>[2x]GPHMSDHKFLTQAVEEAYKGVDCGDGGPFGAVIVHNNEVVASCHNMVLKYTDPTAHAEVTAIREACK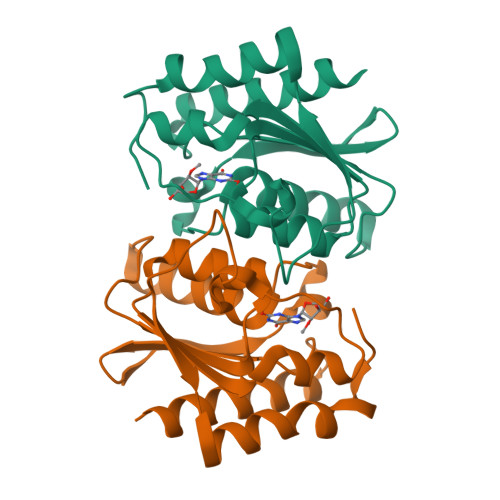KLNKIELSECEIYASCEPCPMCFGAIHLSRLKRLVYGAKAEAAIAIGFDDFIADALRGTGVYQKSSLEIKKADGNGAAIAEQVFQNTKEKFRLY> QRKNNNKRWYFTREQLENSPSRRFGLDPDKELSYRQQAANLLQDMGQRLNVSQLTINTAIVYMHRFYMIQSFTRFHRNSVAPAALFLAAKVEEQPKKLEHVIKVAHTCLHPQESLPDTRSEAYLQQVQDLVILESIILQTLGFELTIDHPHTHVVKCTQLVRASKDLAQTSYFMATNSLHLTTFSLQYTPPVVACVCIHLACKWSNWEIPVSTDGKHWWEYVDATVTLELLDELTHEFLQILEKT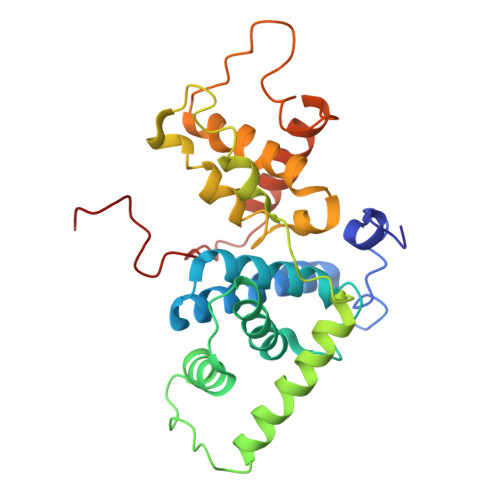PNRLKRIWNWRACQAAKKT>[2x]GAMEKPTNYSQETIASIAQKYQKLAEDINKDRKNNIADQTVIYLLSESLSDPDRVSNVTVSHDVLPNIKAIKNSTTAGLMQSDSYGGGTANMEFQTLTSLPFYNFSSSVSVLYSEVFPKMAKPHTISEFYQGKNRIAMHPASANNFNRKTVYSNLGFSKFLALSGSKDKFKNIENVGLLTSDKTVYNNILSLINPSESQFFSVITMQNHIPWSSDYPEEIVAEGKNFTEEENH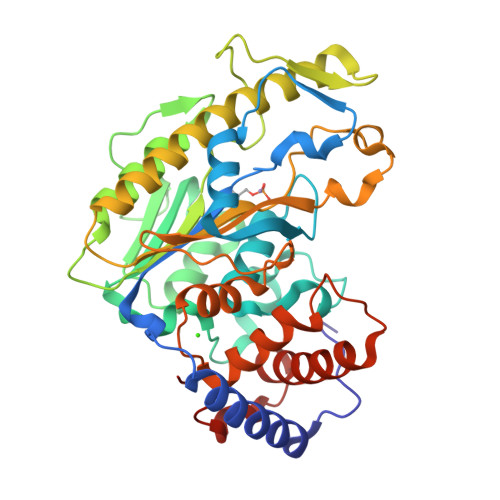NLTSYARLLSFTDKETRAFLEKLTQINKPITVVFYGDHLPGLYPDSAFNKHIENKYLTDYFIWSNGTNEKKNHPLINSSDFTAALFEHTDSKVSPYYALLTEVLNKASVDKSPDSPEVKAIQNDLKNIQYDVTIGKGYLLKHKTFFKISR>MSNEYDEYIANHTDPVKAINWNVIPDEKDLEVWDRLTGNFWLPEKIPVSNDIQSWNKMTPQEQLATMRVFTGLTLLDTIQGTVGAISLLPDAETMHEEAVYTNIAFMESVHAKSYSNIFMTLASTPQINEAFRWSEENENLQRKAKIIMSYYNGDDPLKKKVASTLLESFLFYSGFYLPMYLSSRAKLTNTADIIRLIIRDESVHGYYIGYKYQQGVKKLSEAEQEEYKAYTFDLMYDLYENEIEYTEDIYDDLGWTEDVKRFLRYNANKALNNLGYEGLFPTDETKVSPAI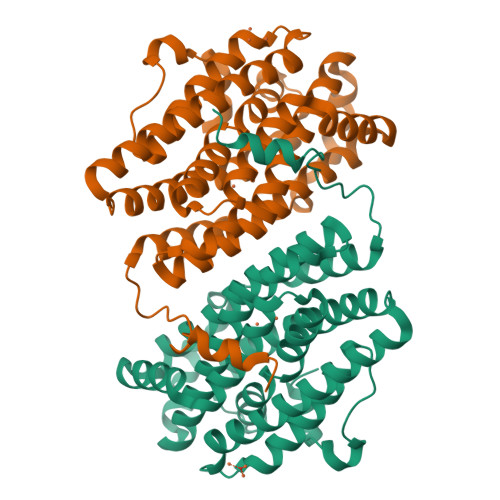LSSLSPNADENHDFFSGSGSSYVIGKAEDTTDDDWDF[4x]>XAAAAALAAALAQALX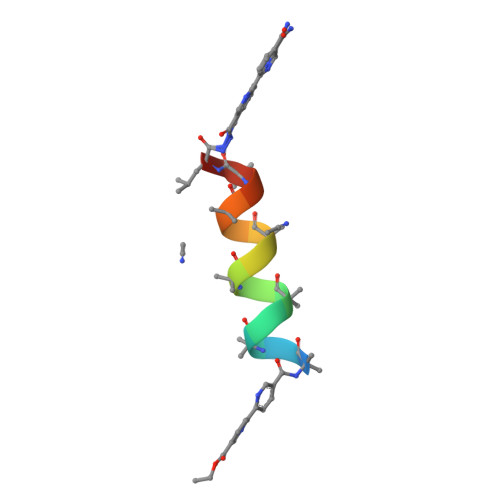[2x]N-methyl-4-{[4-(1-propyl-1H-pyrazol-4-yl)-7H-pyrrolo[2,3-d]pyrimidin-2-yl]amino}benzamide | C20 H21 N7 O 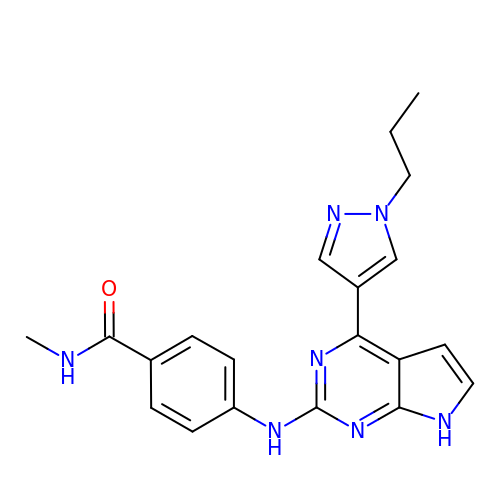| FLBLXKNWKAGVEB-UHFFFAOYSA-N>[2x]KCTKNALAQTGFNKDKYFNGDVWYVTDYLDLEPDDVPKRYCAALAAGTASGKLKEALYHYDPKTQDTFYDVSELQEESPGKYTANFKKVEKNGNVKVDV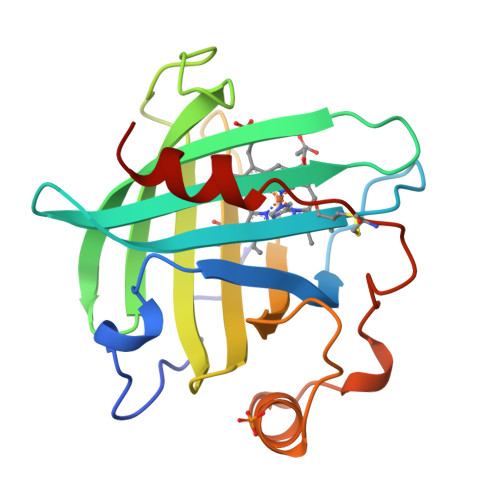TSGNYYTFTVMYADDSSALIHTCLHKGNKDLGDLYAVLNRNKDTNAGDKVKGAVTAASLKFSDFISTKDNKCEYDNVSLKSLLTK> GHMHGRLKVKTSEEQAEAKRLEREQKLKLYQSATQAVFQKRQAGELDESVLELTSQILGANPDFATLWNCRREVLQHLETEKSPEESAALVKAELGFLESCLRVNPKSYGTWHHRCWLLSRLPEPNWARELELCARFLEADERNFHCWDYRRFVAAQAAVAPAEELAFTDSLITRNFSNY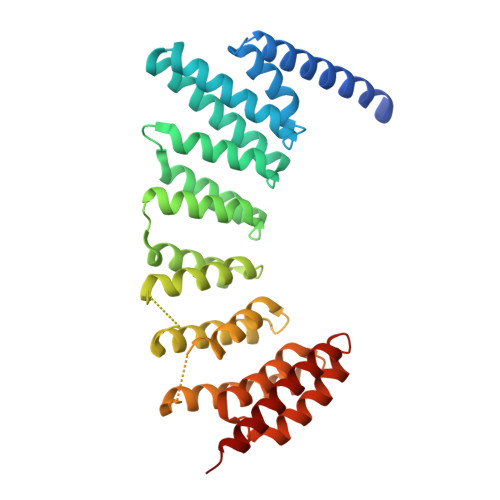SSWHYRSCLLPQLHPQPDSGPQGRLPENVLLKELELVQNAFFTDPNDQSAWFYHRWLLGAGSGRCELSVEKSTVLQSELESCKELQELEPENKWCLLTIILLMRALDPLLYEKETLQYFSTLKAVDPMRAAYLDDLRSKFLLENSVLKMEYA> MSTSTYALRAGKRDVRREQQEIITRQINTAPYVQDAMMRVVVFAQYPSGRYKAFDYVFPDYLKVFLNWRELLEGSGRYPMGVIVSFNGNIDWTRARVEATNMHGLNNTDWREARAWGPHVICGNQLRKAGHLSRAVYVPLDEHNTVKVLATARQDGALNRFNGPQLAQTLTNNIVCPNVIEFNTESDVIDYAKMAHIAYIDQAGLIVASSDAYISGDSQA

Cypoviruses, members of the family Reoviridae, subfamily Spinareovirus, possess a single capsid layer with turrets and are commonly embedded in crystalline occlusion bodies called polyhedra, which are formed in the cell cytoplasm and mainly composed of a single virus-encoded protein, polyhedrin. To ensure the delivery of virus particles to the target intestinal cells, allowing the transmission of packages of infectious virus between hosts by oral-faecal routes, polyhedra are disrupted only when they are exposed to the very alkaline pH environment found in insect midguts. The fold of all the polyhedrins is highly similar – a β-barrel core sitting on a base domain, surrounded by a common array of five helices (H1–H5). The strongest intermolecular interactions define a trimer composed of a cluster of three β-barrels sandwiched by helices top and bottom.

Base domain deletion mutants of CPV1 (CPV1Δ) and CPV4 (CPV4Δ) were produced by three steps of PCR using primers encoding a Gly-Ser-Gly linker (described in). To test this, polyhedrin proteins were made with the base domain removed by deleting residues 74–110 of CPV4 and 71–103 of CPV1 and replacing them with a flexible Gly-Ser-Gly linker (resulting in CPV4Δ and CPV1Δ respectively). The CPV4Δ structure was very similar to that of CPV4 with the larger unit cell. The absence of the base domain did not influence the overall structure of the trimeric building block but increased flexibility such that the electron density for 40–50 residues in the inter-trimer contact areas could not be observed. The base domain is therefore a region that is neither required for proper folding of the protein, nor for crystal assembly, but fine-tunes the crystal, ‘locking-down’ the structure, often in conjunction with NTPs. In contrast in the base domain deletion mutants all major cavities are connected, resulting in contiguous solvent channels running through the crystal lattice. The deletion mutants are much more sensitive to alkaline buffers, even those such as glycine and borate which do not disrupt crystals of full-length polyhedrin, although CAPS could not dissolve any of the samples effectively. We also find that the whole base domain is dispensable for polyhedra formation, although the biochemical features are altered dramatically when it is removed.The asymmetric outer membrane (OM) comprises phospholipids in the inner leaflet and lipopolysaccharide (LPS) in the outer leaflet and is essential for Gram-negative bacteria. LptB hydrolyzes ATP to provide energy for LPS extraction and transport. To understand the structural basis of how ABC transporter LptB2FG extracts and transports LPS, we have solved the crystal structure of the LptB2FG complex from Klebsiella pneumoniae.

The structure was determined to a resolution of 3.7 Ångström (Å) by the single-wavelength anomalous dispersion (SAD) using data sets collected at 1.0723 Å, and the sequence register was validated using sulfur anomalous data and selenomethionine anomalous data. Heavy-atom derivatives were obtained by soaking the crystals in potassium tetranitroplatinate (II) (see “Methods” section). LptF and LptG each contain six α-helical transmembrane segments, namely TM1-6-F and TM1-6-G, respectively, a periplasmic β-jellyroll domain, three periplasmic loops, and a pair of cytoplasmic turns. LptF and LptG form a hetero-dimeric cavity with a total of 12 TM segments and the two LptB copies form a homo-dimer in a “V” shape at the cytoplasmic face of the TMDs region. Overall, the dimension of the LptB2FG transporter is of ~86 Å in width and 128 Å in length. The two periplasmic β-jellyroll domains are shifted to one side of the transporter thus generating a periplasmic opening at the side of the TM5F-TM1G interface. The IM section of the internal cavity is very hydrophobic, while the section above the IM is highly positively charged. There is an extra electron density in the cavity that could not be assigned with any confidence. The highly conserved residues K34 (TM1G) and R136 (TM3G) of LptG are found at the upper cavity of the transporter and around this extra electron density. The periplasmic domains of LptF and LptG adopt β-jellyroll folds, which together comprise 10 β-strands in a manner that resembles the periplasmic β-jellyroll domain of LptC.

>MATLTAKNLAKAYKGRRVVEDVSLTVNSGEIVGLLGPNGAGKTTTFYMVVGIVPRDAGNIIIDDEDISLLPLHARARRGIGYLPQEASIFRRLSVYDNLMAVLQIRDDLTSEQREDRAKELMEEFHIEHLRDSLGQALSGGERRRVEIARALAANPKFILLDEPFAGVDPISVIDIKRIIEHLRDSGLGVLITDHNVRETLAVCERAYIVSQGHLIAHGTPQQILEDEQVKRVYLGEDFRL[2x];> MIIIRYLVRETLKSQLAILFILLLIFFCQKLVRILGAAVDGDIPTNLVLSLLGLGIPEMAQLILPLSLFLGLLMTLGKLYTESEITVMHACGLSKAVLIKAAMILAVFTGAVAAVNVMWAGPWSSRHQDEVLAEAKANPGMAALAQGQFQQASDGNAVMFIESVNGNRFHDVFLAQLRPKGNARPSVVVADSGELSQQKDGSQYVTLNKGTRFEGTAMLRDFRITDFNNYQAIIGHQAVSADPDDTEQMDMRTLWKTHTDRARAELHWRFTLVATVFIMALMVVPLSVVNPRQGRVLSMLPAMLLYLVFFLLQTSIKSNGGKGKMDPAIWMWAINLLYFALAVLLNLWDTVPMRRFRARFNKGAA;> MQAFGVLDRYIGKTIFNTIMMTLFMLVSLSGIIKFVDQLKKSGQGSYDALGAGLYTILSVPKDIQIFFPMAALLGALLGLGMLAQRSELVVMQASGFTRLQVALAVMKTAIPLVLLTMAIGEWVAPQGEQMARNYRAQQMYGGSLLSTQQGLWAKDGHNFVYIERVKGNDELGGVSIYAFNPERRLQSVRYAASAKFDSENKVWRLSQVDESDLTDPKQVTGSQMVSGTWKTNLTPDKLGVVALDPDALSISGLHNYVKYLKSSGQDPGRYQLNMWSKIFQPLSVAVMMLMALSFIFGPLRSVPMGVRVVTGISFGFIFYVLDQIFGPLTLVYGIPPIIGALLPSASFFLISLWLMMRKA Tumor-suppressor let-7 pre-microRNAs (miRNAs) are regulated by terminal uridylyltransferases TUT7 and TUT4 that either promote let-7 maturation by adding a single uridine nucleotide to the pre-miRNA 3′ end or mark them for degradation by the addition of multiple uridines. Oligo-uridylation is increased in cells by enhanced TUT7/4 expression and especially by the RNA-binding pluripotency factor LIN28A. TUT4 and TUT7 are multidomain enzymes whose specific targeting of RNAs makes use of three zinc fingers, combined with two copies of a nucleotidyltransferase domain (NTD), one inactive in the N-terminal half of the polypeptide (pseudo-NTD) and one active in the C-terminal half. Our structures reveal that pre-miRNAs engage the enzymes in fundamentally different ways depending on the presence of LIN28A, which clamps them onto the TUTs to enable processive 3′ oligo-uridylation.

To visualize the TUT7 apo state we initially isolated the enzyme bound with UTPαS alone but found that modification with NHS-polyethyleneglycol4 (NHS-PEG4)39 was needed to avert excessive sticking of particles to the air–water interface where they are prone to denaturation. The TUT7 structure in an apo state at 4.03 Å revealed an overall ‘C-shape’ conformation composed of two right-handed conformers distinct from the ‘L-shape’ of human Dicer, which in addition remains similar in its conformation throughout its activity cycle. This difference suits Dicer’s role as a ‘tape-measure’ protein capable of recognizing the length associated with a correctly generated pre-miRNA, hence its need for a fixed dimension, whereas the TUTs need to be able to function in two different modes (mono- and oligo-uridylation) and, further, to be able to act processively on a bound pre-miRNA substrate under the influence of LIN28A. In both the apo state and the binary TUT7 complex the two NTDs maintain the distinctive ‘C-shape’, apparently due to their direct interaction with one another. By contrast, in the apo state no obvious density was resolved for the backbone link connecting the LIM and CM, with only a small region of the linking density visible associated with the LIM. Nevertheless, for maintenance of the distinctive ‘C-shape’ structure, the two NTDs of the enzyme must still be interacting directly in the apo state, albeit relatively weakly. After binding to pre-let-7g/LIN28A, the zinc finger in the TUT7 LIM was observed with good density, whereas it was unobserved in TUT7 apo or binary states because of mobility and/or disorder.

> MGDTAKPYFVKRTKDRGTMDDDDFRRGHPQQDYLIIDDHAKGHGSKMEKGLQKKKITPGNYGNTPRKGPCAVSSNPYAFKNPIYSQPAWMNDSHKDQSKRWLSDEHTGNSDNWREFKPGPRIPVINRQRKDSFQENEDGYRWQDTRGCRTVRRLFHKDLTSLETTSEMEAGSPENKKQRSRPRKPRKTRNEENEQDGDLEGPVIDESVLSTKELLGLQQAEERLKRDCIDRLKRRPRNYPTAKYTCRLCDVLIESIAFAHKHIKEKRHKKNIKEKQEEELLTTLPPPTPSQINAVGIAIDKVVQEFGLHNENLEQRLEIKRIMENVFQHKLPDCSLRLYGSSCSRLGFKNSDVNIDIQFPAIMSQPDVLLLVQECLKNSDSFIDVDADFHARVPVVVCREKQSGLLCKVSAGNENACLTTKHLTALGKLEPKLVPLVIAFRYWAKLCSIDRPEEGGLPPYVFALMAIFFLQQRKEPLLPVYLGSWIEGFSLSKLGNFNLQDIEKDVVIWEHTDSAAGDTGITKEEAPRETPIKRGQVSLILDVKHQPSVPVGQLWVELLRFYALEFNLADLVISIRVKELVSRELKDWPKKRIAIEDPYSVKRNVARTLNSQPVFEYILHCLRTTYKYFALPHKITKSSLLKPLNAITCISEHSKEVINHHPDVQTKDDKLKNSVLAQGPGATSSAANTCKVQPLTLKETAESFGSPPKEEMGNEHISVHPENSDCIQADVNSDDYKGDKVYHPETGRKNEKEKVGRKGKHLLTVDQKRGEHVVCGSTRNNESESTLDLEGFQNPTAKECEGLATLDNKADLDGESTEGTEELEDSLNHFTHSVQGQTSEMIPSDEEEEDDEEEEEEEEPRLTINQREDEDGMANEDELDNTYTGSGDEDALSEEDDELGEAAKYEDVKECGKHVERALLVELNKISLKEENVCEEKNSPVDQSDFFYEFSKLIFTKGKSPTVVCSLCKREGHLKKDCPEDFKRIQLEPLPPLTPKFLNILDQVCIQCYKDFSPTIIEDQAREHIRQNLESFIRQDFPGTKLSLFGSSKNGFGFKQSDLDVCMTINGLETAEGLDCVRTIEELARVLRKHSGLRNILPITTAKVPIVKFFHLRSGLEVDISLYNTLALHNTRLLSAYSAIDPRVKYLCYTMKVFTKMCDIGDASRGSLSSYAYTLMVLYFLQQRNPPVIPVLQEIYKGEKKPEIFVDGWNIYFFDQIDELPTYWSECGKNTESVGQLWLGLLRFYTEEFDFKEHVISIRRKSLLTTFKKQWTSKYIVIEDPFDLNHNLGAGLSRKMTNFIMKAFINGRRVFGIPVKGFPKDYPSKMEYFFDPDVLTEGELAPNDRCCRICGKIGHFMKDCPMRRKVRRRRDQEDALNQRYPENKEKRSKEDKEIHNKYTEREVSTKEDKPIQCTPQKAKPMRAAADLGREKILRPPVEKWKRQDDKDLREKRCFICGREGHIKKECPQFKGSSGSLSSKYMTQGKASAKRTQQES> MRISERAFMDIAIGTKAPRRIVFKLFPRKCPSAVKNFIELCSGNVSTDTYESGN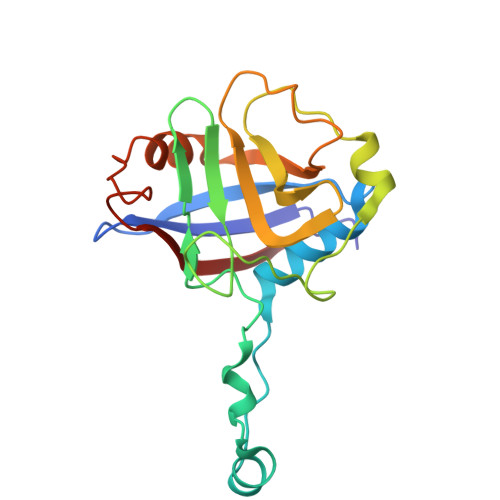RDKLISESALPQLTYKNSTFHRVEKGYLIQGGDIVTGRGTEQLSIYGGTFSAPEEVRASVFDKPGLVGTASSSPNAHGSQFFILTAKEANHLNGTCICFGQVADGLDVVQEIEQVPIDPSGFPSLKVSIVDCGVLE> DREKIYQWINELSSPETRENALLELSKKRESVPDLAPM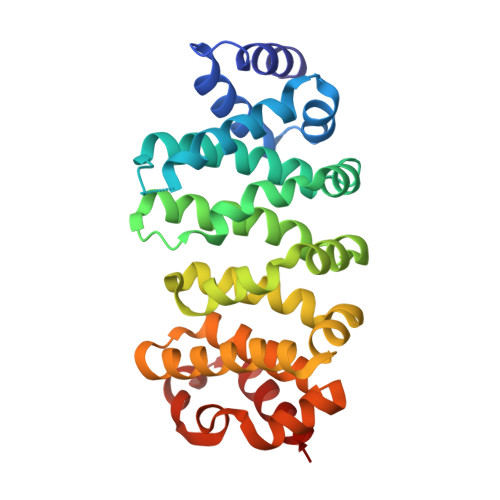LWHSFGTIAALLQEIVNIYPSINPPTLTAHQSNRVCNALALLQCVASHPETRSAFLAAHIPLFLYPFLHTVSKTRPFEYLRLTSLGVIGALVKTDEQEVINFLLTTEIIPLCLRIMESGSELSKTVATFILQKILLDDTGLAYICQTYERFSHVAMILGKMVLQLSKEPSARLLKHVVRCYLRLSDNPRAREALRQCLPDQLKDTTFAQVLKDDTTTKRWLAQLVKNLQ2-deoxy-2-fluoro-beta-D-mannopyranosyl fluoride | C6 H10 F2 O4 | 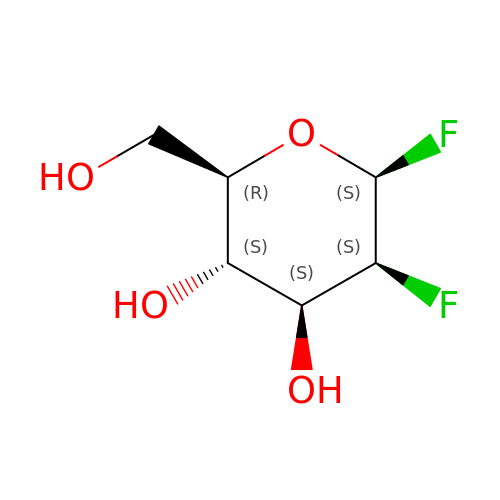YZRDPODBASCWCK-CBPJZXOFSA-N3-(quinazolin-4-ylsulfanyl)propanoic acid 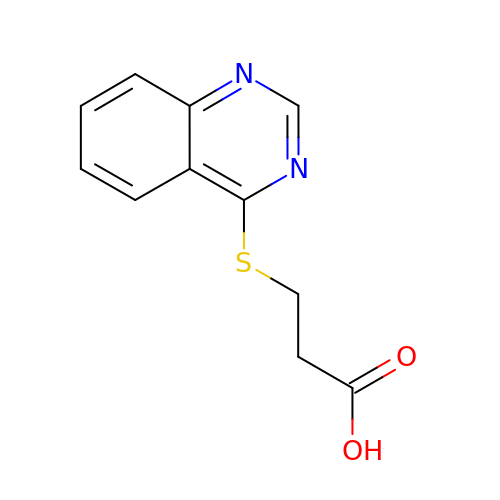| C11 H10 N2 O2 S | WQTFNWOAHQIRIR-UHFFFAOYSA-N>VKLAGNSSLCPINGWAVYSKDNSIRIGSKGDVFVIREPFISCSHLECRTFFLTQGALLNDKHSNGTVKDRSPHRTLMSCPVGEAPSPYNSRFESVAWSASACHDGTSWLT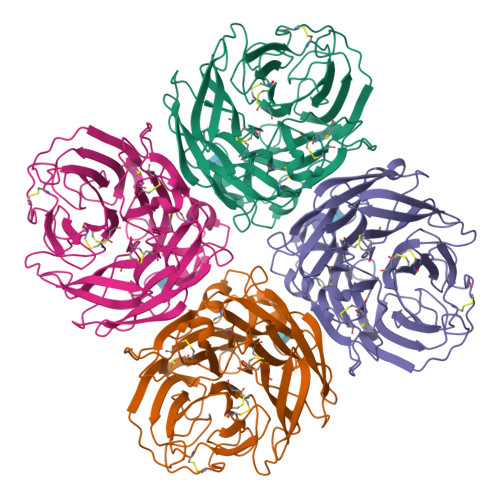IGISGPDNGAVAVLKYNGIITDTIKSWRNNILRTQESECACVNGSCFTVMTDGPSNGQASYKIFKMEKGKVVKSVELDAPNYHYEECSCYPNAGEITCVCRDNWHGSNRPWVSFNQNLEYQIGYICSGVFGDNPRPNDGTGSCGPVSSNGAYGVKGFSFKYGNGVWIGRTKSTNSRSGFEMIWDPNGWTETDSSFSVKQDIVAITDWSGYSGSFVQHPELTGLDCIRPCFWVELIRGRPKESTIWTSGSSISFCGVNSDTVGWSWPDGAELPFTIDK[8x]6-DEOXYERYTHRONOLIDE B | C21 H38 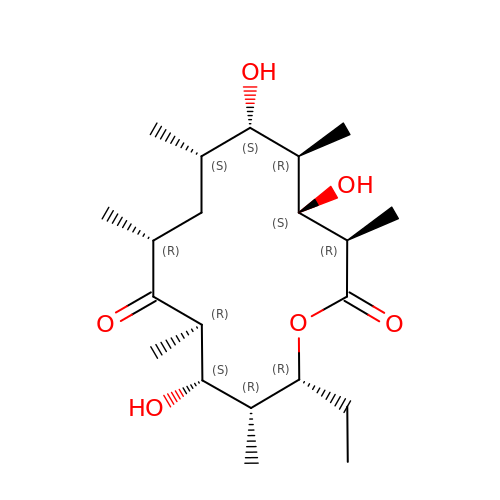O6 | HQZOLNNEQAKEHT-IBBGRPSASA-N> MGSDKIHHHHHHMSKTLKEITDQKNELKK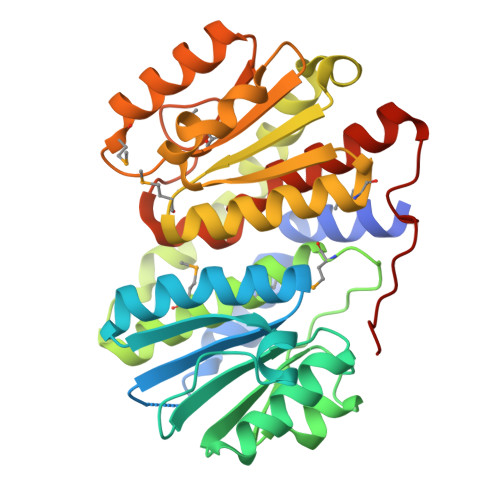FFENFVLNLEKTEIFSEIQKNLTDEVLFVGCGSSYNLALTISYYFERVLKIRTKAIPAGEVAFQKIPDLEERGLAFLFSRTGNTTEVLLANDVLKKRNHRTIGITIEEESRLAKESDLPLVFPVREEAIVMTKSFSMILLSLMFLADKIAGNSTERFSELVGYSPEFFDISWKVIEKIDLKEHDHFVFLGMSEFFGVSLESALKCIEMSLTFSEAYSTLEYRHGPKALVKKGTLVFMQKVSGMDEQEKRLRKELESLGATVLEVGEGGDIPVSNDWKSAFLRTVPAQILGYQKAISRGISPDKPPHLEKTVVL S-3-(4-FLUOROPHENOXY)-2-HYDROXY-2-METHYL-N-[4-NITRO-3-(TRIFLUOROMETHYL)PHENYL]PROPANAMIDE | C17 H14 F4 N2 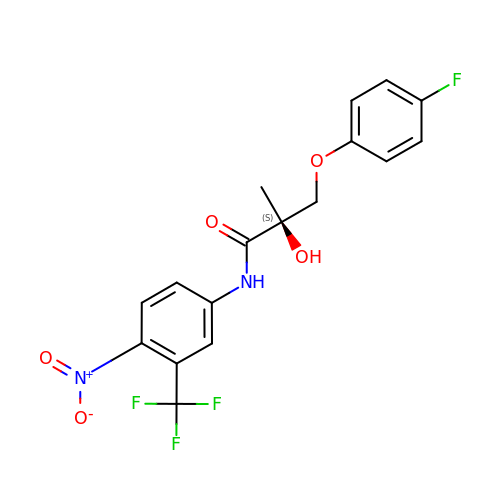O5 | KJMFOTCDISOHDX-INIZCTEOSA-N>MAKKTSSKGKLPPGPLPLPGLGNLLHVDFQNTPYCFDQLRRRFGDVFSLQLAWTPVVVLNGLAAVREALVTHGEDTADRPPVPITQILGFGPRSQGVFLARYGPAWREQRRFSVSTLRNLGLGKKSLEQWVTEEAACLCAAFANHSGRPFRPNGLLDKAVSNVIASLTCGRRFEYDDPRFLRLLDLAQEGLKEESGFLREVLNAVPVLLHIPALAGKVLRFQKAFLTQLDELLTEHRMTWDPAQPPRDLTEAFLAEMEKAKGNPESSFNDENLRIVVADLFSAGMETTSTTLAWGLLLMILHPDVQRRVQ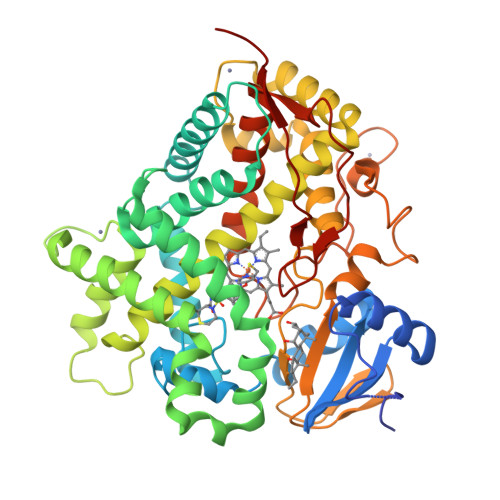QEIDDVIGQVRRPEMGDQAHMPYTTAVIHEVQRFGDIVPLGVTHMTSRDIEVQGFRIPKGTTLITNLSSVLKDEAVWEKPFRFHPEHFLDAQGHFVKPEAFLPFSAGRRACLGEPLARMELFLFFTSLLQHFSFSVPTGQPRPSHHGVFAFLVSPSPYELCAVPRHHHH[2x]>[2x]GMPRAAVVCGLGSYLPEAVLSNDMLAAELDTSDAWISSRTGVR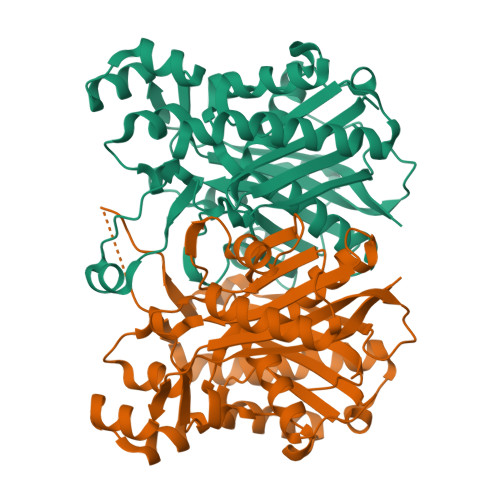QRHIAGDLGSGDLALRAASAALASAGLERVDAVVLATSTGDFCCPATAPRVAARLGLVGALAFDLSAAATGFVYGLASVGSLISAGLADSALLVGVDTFSHTLDPADRSTRALFGDGAGAVVLRAGDAEEEGALLAFDLGSDGHQFDLLMTPAVSRAERSSGQASNYFRMDGKAVFGQAVTQMSDSVRRVLDRVGWQASDLHHLVPHQANTRILAAVADQLDLPVERVVSNIAEVGNTVAASIPLALAHGLRQGILRDGGNMVLTGFGAGLTWGSVALRWPKIVPTMD>[2x]NRILPDSVDWREKGCVTEVKYQGSCGACWAFSAVGALEAQLKLKTGK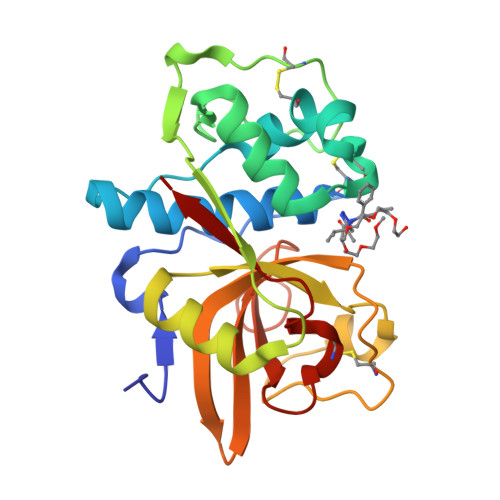LVSLSAQNLVDCSTEKYGNKGCNGGFMTTAFQYIIDNKGIDSDASYPYKAMDQKCQYDSKYRAATCSKYTELPYGREDVLKEAVANKGPVSVGVDARHPSFFLYRSGVYYEPSCTQNVNHGVLVVGYGDLNGKEYWLVKNSWGHNFGEEGYIRMARNKGNHCGIASFPSYPEI>[4x]GSHMASAVAVDLGNRKLEISSGKL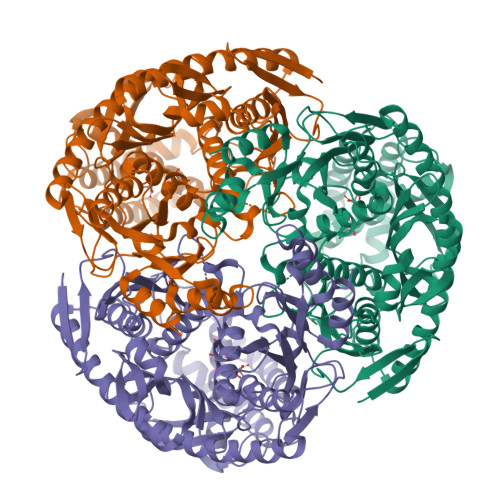ARFADGSAVVQSGDTAVMVTAVSKTKPSPSQFMPLVVDYRQKAAAAGRIPTNYLRREVGTSDKEILTSRIIDRSIRPLFPAGYFYDTQVLCNLLAVDGVNEPDVLAINGASVALSLSDIPWNGPVGAVRIGIIDGEYVVNPTRKEMSSSTLNLVVAGAPKSQIVMLEASAENILQQDFCHAIKVGVKYTQQIIQGIQQLVKETGVTKRTPQKLFTPSPEIVKYTHKLAMERLYAVFTDYEHDKVSRDEAVNKIRLDTEEQLKEKFPEADPYEIIESFNVVAKEVFRSIVLNEYKRCDGRDLTSLRNVSCEVDMFKTLHGSALFQRGQTQVLCTVTFDSLESGIKSDQVITAINGIKDKNFMLHYEFPPYATNEIGKVTGLNRRELGHGALAEKALYPVIPRDFPFTIRVTSEVLESNGSSSMASACGGSLALMDSGVPISSAVAGVAIGLVTKTDPEKGEIEDYRLLTDILGIEDYNGDMDFKIAGTNKGITALQADIKLPGIPIKIVMEAIQQASVAKKEILQIMNKTISKPRASRKENGPVVETVQVPLSKRAKFVGPGGYNLKKLQAETGVTISQVDEETFSVFAPTPSAMHEARDFITEICK> MIQLFDYYNQETQDLHDSLLAAGYACPTIVIEANGFLPDDMISPYTYFLGDEEGVDHPLFFNQVPVPPFWEITGDHQVARVSDMGEERARIHYASQARGRLVKQVDWLDKKGQLRLSERYNKQGRCFAKTAYKSGQEAFNTTYYSTDGQERIVENHVTGDIILTLDQEPLRIFKSRV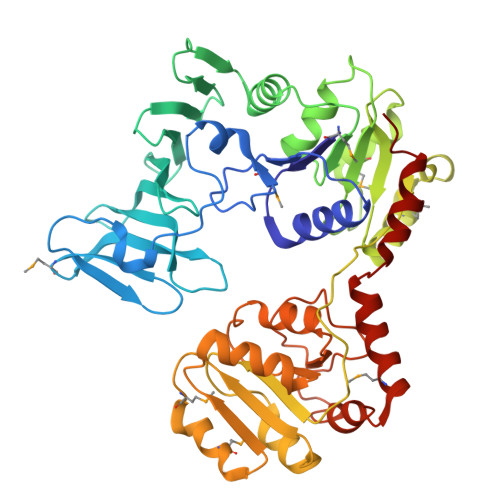DFIRFFLERLDLDLDHILFNSLAYSFLVSHSLTGRAGQDILFWQEPLYDELPGNMQLILDNSQLRTQTIVIPDLATYEKAMSLAAADQQQKFLHLGYHYDFKRDNYLRKDALILTHSDQIEGLDTLVQSLPQLVFRIAALTEMSPKLLSMLSYKNVVLYQNASLKQIEQLYLESDIYLDINHGGQVLQAVRKAFENNLLILGFEQTLHDRHYIAQQHIFDSSQPAQLASILEEALCGVEQMRSALQAQGRHANDVPVSLYQETLQSLLGG>MEVSPLQPVNENMQVNKIKKNEDAKKRLSVERIYQKKTQLEHILLRPDTYIGSVELVTQQMWVYDEDVGINYREVTFVPGLYKIFDEILVNAADNKQRDPKMSCIRVTIDPENNLISIWNNGKGIPVVEHKVEKMYVPALIFGQLLTSSNYDDDEKKVTGGRNGYGAKLCNIFSTKFTVETASREYKKMFKQTWMDNMGRAGEMELKPFNGEDYTCITFQPDLSKFKMQSLDKDIVALMVRRAYDIAGSTKDVKVFLNGNKLPVKGFRSYVDMYLKDKLDETGNSLKVIHEQVNHRWEVCLTMSEKGFQQISFVNSIATSKGGRHVDYVADQIVTKLVDVVKKKNKGGVAVKAHQVKNHMWIFVNALIENPTFDSQTKENMTLQPKSFGSTCQLSEKFIKAAIGCGIVESILNWVKFKAQVQLNKKCSAVKHNRIKGIPKLDDANDAGGRNSTECTLILTEGDSAKTLAVSGLGVVGRDKYGVFPLRGKILNVREASHKQIMENAEINNIIKIVGLQYKKNYEDEDSLKTLRYGKIMIMTDQDQDGSHIKGLLINFIHHNWPSLLRHRFLEEFITPIVKVSKNKQEMAFYSLPEFEEWKSSTPNHKKWKVKYYKGLGTSTSKEAKEYFADMKRHRIQFKYSGPEDDAAISLAFSKKQIDDRKEWLTNFMEDRRQRKLLGLPEDYLYGQTTTYLTYNDFINKELILFSNSDNERSIPSMVDGLKPGQRKVLFTCFKRNDKREVKVAQLAGSVAEMSSYHHGEMSLMMTIINLAQNFVGSNNLNLLQPIGQFGTRLHGGKDSASPRYIFTMLSSLARLLFPPKDDHTLKFLYDDNQRVEPEWYIPIIPMVLINGAEGIGTGWSCKIPNFDVREIVNNIRRLMDGEEPLPMLPSYKNFKGTIEELAPNQYVISGEVAILNSTTIEISELPVRTWTQTYKEQVLEPMLNGTEKTPPLITDYREYHTDTTVKFVVKMTEEKLAEAERVGLHKVFKLQTSLTCNSMVLFDHVGCLKKYDTVLDILRDFFELRLKYYGLRKEWLLGMLGAESAKLNNQARFILEKIDGKIIIENKPKKELIKVLIQRGYDSDPVKAWKEAQQKVPDEEENEESDNEKETEKSDSVTDSGPTFNYLLDMPLWYLTKEKKDELCRLRNEKEQELDTLKRKSPSDLWKEDLATFIEELEAVEAKEKQDEQVGLPGKGGKAKGKKTQMAEVLPSPRGQRVIPRITIEMKAEAEKKNKKKIKNENTEGSPQEDGVELEGLKQRLEKKQKREPGTKTKKQTTLAFKPIKKGKKRNPWSDSESDRSSDESNFDVPPRETEPRRAATKTKFTMDLDSDEDFSDFDEKTDDEDFVPSDASPPKTKTSPKLSNKELKPQKSVVSDLEADDVKGSVPLSSSPPATHFPDETEITNPVPKKNVTVKKTAAKSQSSTSTTGAKKRAAPKGTKRDPALNSGVSQKPDPAKTKNRRKRKPSTSDDSDSNFEKIVSKAVTSKKSKGESDDFHMDFDSAVAPRAKSVRAKKPIKYLEESDEDDLF[2x]

The human type IIA topoisomerases (Top2) are essential enzymes that regulate DNA topology and chromosome organization. The passage of the T-segment requires ATP hydrolysis and is thought to occur along with the opening and closing of several dimeric interfaces constituting molecular gates. In this work, we determined the cryo-EM structure of the full-length human Topo IIα isoform bound to DNA in different conformations trapped by the anti-cancer drug etoposide.

Each particle stack was submitted to 3D heterogeneous classification and refinement without mask to yield two reconstructions of the entire complex in State 1 at 4.7 Å resolution from 26,506 particles, and in State 2 at 7.4 Å resolution from 13,420 particles. The 27-aa linkers between the two domains, missing from the crystal structure of the isolated ATPase domain, were built as alpha helices based on secondary structure predictions and using well-defined linker densities of the cryo-EM map obtained by focused classification on the ATPase domain. Finally, the atomic model of the DNA-binding/cleavage domain in State 2 and the corresponding full-length hTopo IIα in State 2 were refined using State 1 model as a reference. We also found that the ATPase domain adopts different inclinations depending on the conformation of the DNA-binding/cleavage domain. In the pre-open state, the ATPase domain can bend over by about 15°. In the closed state, the distance between the two residues N433 is 49.3 Å while the distance is shortened to 46.4 Å in the pre-open state. Consequently, this translational movement of 3 Å in the orthogonal plane of the DNA gate induces the rotation of the ATPase domain by 12° counterclockwise, opposite to the intertwining. It also forces the ATPase domain to come closer to the DNA-gate prefiguring a conformation that would position the T-segment in the newly formed groove between the TOPRIM and tower domains. Altogether the rotation of the N-gate that correlates with the oscillation of the DNA-gate can be associated with a corkscrew mechanism that we can extrapolate from the two overall conformations of the full-length catalytic core.> MSEKTVLSIQSFVTHGYVGNKAATFPLQLHGFDVDGINTVCLSNHSGYPVIRGHRMSLQEYDELMEGVRANNFLSNYRYILTGYINNVDIIGRIRDTLKEVRELREKEDKKLTFICDPVMGDDGIMYCKKEVLDAYRELVPLADIVTPNYFEASLLSGVTVNDLSSAILAADWFHNCGVAHVIIKSFREQENPTHLRFLYSVKEGSEAAVRRFSGVVPYHEGRYTGTGDVFAACLLAFSHSHPMDVAIGKSMAVLQELIIATRKEGGDGKSSLKSRELRVVASPQVVLQPSTVVDVKPIS

In the salvage pathway, extracellular PLP is first converted to pyridoxal (PL) by non-specific alkaline phosphatases, then PL or the B6 vitamers, pyridoxine (PN) and pyridoxamine (PM), are taken up into cells where they are phosphorylated by the enzyme pyridoxal kinase (PdxK). Genome analysis suggests that trypanosomatids, including the African trypanosome T. brucei, lack genes for de novo biosynthesis of vitamin B6 and are therefore dependent on the salvage pathway, particularly PdxK, for the production of PLP. The genetic studies presented here clearly demonstrate that pyridoxal kinase activity is essential for growth and survival of Trypanosoma brucei in vitro and in vivo. The resulting structure revealed that TbPdxK has a typical ribokinase central core of β-sheets surrounded by α-helices.

The secondary structure of each monomer comprises a 6-stranded parallel central β-sheet (strands 1, 2, 5, 6, 7, 8), a 2-stranded anti-parallel β-sheet (strands 3 and 4), and a 3-stranded anti-parallel β-sheet (strands 9, 10, 11). These are flanked by four α-helices on one side and 3 on the other. Two loops (120–129, and 266–274) are missing from the model due to their flexibility and resulting lack of electron density, and several amino acids had to be truncated to alanine residues in the model as a result of side-chain flexibility (Lys99, Lys130, Glu131, Arg188, Arg223, Glu265 and Ser275). The crystal structure of TbPdxK shows that the ATP takes on two alternate conformations in this crystal form. Compared with the human and sheep ATP-bound form, the adenine ring is rotated through 90° resulting in different protein contacts. The TbPdxK adenine amine interacts with His220 carbonyl while in the human and sheep enzymes the interactions are with Val226, Ala228, and Phe230 backbone atoms (the latter via a water molecule). In the two different ATP binding modes of TbPdxK, the γ-phosphates make different interactions. In one conformation, the γ-phosphate interacts with Asp117 and Glu152, as seen in human and E. coli PdxK. In the second conformation, the interactions are with Thr227, as in sheep PdxK, and backbone atoms of Tyr224 and Gly228. The conserved GTGD ribokinase motif is present in the TbPdxK amino acid sequence (residues 226–229), and is seen in this structure to bind the γ-phosphate as in sheep PdxK, rather than the α-phosphate as seen for human and E. coli.In plant biosynthesis, the formation of glycosidic bond is usually catalyzed by uridine diphosphate-dependent glycosyltransferases (UGTs). In this work, we report an efficient phenolic apiosyltransferase GuApiGT from G. uralensis, and dissect mechanisms for its sugar donor selectivity towards UDP-Api through crystal structure analysis, theoretical calculations, and mutagenesis. GuApiGT could efficiently and regio-selectively catalyze 2″-O-apiosylation of flavonoid glycosides, and showed strict sugar donor selectivity towards UDP-Api. This selectivity was highly related with the unique 45-amino acid PSPG box and the key RLGSDH sugar binding motif. Through theoretical calculations and rational design, we altered the sugar donor selectivity of GuApiGT and Sb3GT1.

To further prove the critical role of the RLGSDH motif in UDP-Api selectivity, we conducted site-directed mutagenesis of Sb3GT1. It shares 19.8% amino acid sequence identity with GuApiGT. We solved the complex crystal structure of Sb3GT1/UDP at 1.9 Å resolution, and the RMSD compared with GuApiGT is 2.64 Å. The RLGSDH motif in GuApiGT is mapped to FFGDQ of Sb3GT1. Based on structural analysis, we inserted a serine residue into the motif and constructed the 375S/Q377H mutant of Sb3GT1, as well as the F372R/Q376H and F372R/375S/Q377H mutants. All the three mutants could catalyze kaempferol into its 3-O-apioside, according to the characteristic [Y0-H]- ion at m/z 284 in LC/MS analysis.

> MVFQSHIGVLAFPFGTHAAPLLTVVQRLATSSPHTLFSFFNSAVSNSTLFNNGVLDSYDNIRVYHVWDGTPQGQAFTGSHFEAVGLFLKASPGNFDKVIDEAEVETGLKISCLITDAFLWFGYDLAEKRGVPWLAFWTSAQCALSAHMYTHEILKAVGSNGVGETAEEELIQSLIPGLEMAHLSDLPPEIFFDKNPNPLAITINKMVLKLPKSTAVILNSFEEIDPIITTDLKSKFHHFLNIGPSILSSPTPPPPDDKTGCLAWLDSQTRPKSVVYISFGTVITPPENELAALSEALETCNYPFLWSLNDRAKKSLPTGFLDRTKELGMIVPWAPQPRVLAHRSVGVFVTHCGWNSILESICSGVPLICRPFFGDQKLNSRMVEDSWKIGVRLEGGVLSKTATVEALGRVMMSEEGEIIRENVNEMNEKAKIAVEPKGSSFKNFNKLLEIINAPQSS> MTNTLQVKLLSKNARMPERNHKTDAGYDIFSAETVVLEPQEKAVIKTDVAVSIPEGYVGLLTSRSGVSSKTHLVIETGKIDAGYHGNLGINIKNDHEDDKMQT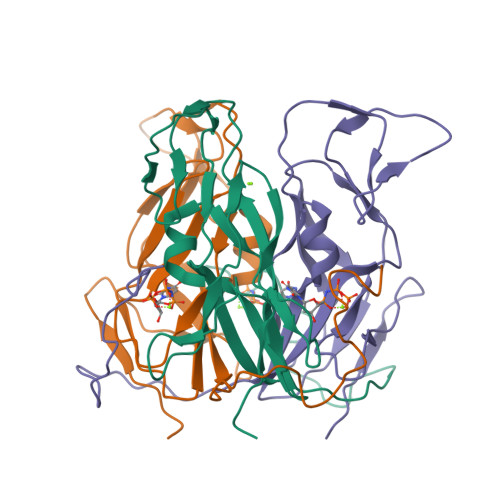IFLRNIDNEKIFEKERHLYKLGSYRIEKGERIAQLVIVPIWTPELKQVEEFESVSERGEKSFGSSGV> METLVRPKPELLKLLKSVGAQKDTYTMKEVLFYLGQYIMTKRLYDEKQQHIVYCSNDLLGDLFGVPSFSVKEHRKIYTMI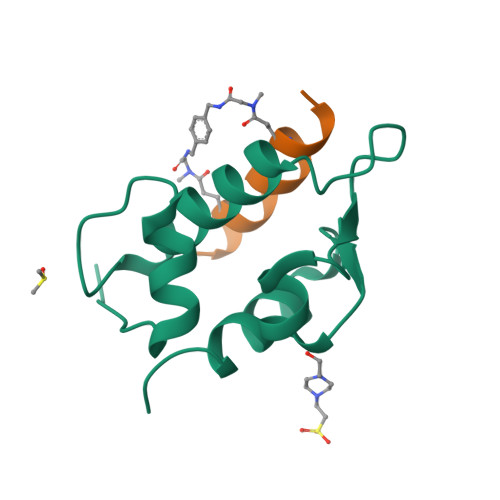YRNLVV;> LTFEQYWAQLESAA>SKDRISWLGQPMKIEENRTYYQKVSIDEEMLEVGDCVSVIPDDSSKPLYLARVTALWEDKNGQMMFHAHWFCAGTDTVLGATSDPLELFLVGECENMQLSYIHSKVKVIYKAPSENWAMEGGTDPETTLPGAEDGKTYFFQLWYNQEYARFESPPKTQPTEDNKHKFCLSCIRLAELRQKEMPKVLEQIEEVDGRVYCSSITKNGVVYRLGDSVYLPPEAFTFNIKVASPVKRPKKDPVNETLYPEHYRKYSDYIKGSNLDAPEPYRIGRIKEIHCGKKKGKVNEADIKLRLYKFYRPENTHRSYNGSYHTDINMLYWSDEEAVVNFSDVQGRCTVEYGEDLLESIQDYSQGGPDRFYFLEAYNSKTKNFEDPPNHARSPGNKGKGKGKGKGKGKHQVSEPKEPEAAIKLPKLRTLDVFSGCGGLSEGFHQAGISETLWAIEMWDPAAQAFRLNNPGTTVFTEDCNVLLKLVMAGEVTNSLGQRLPQKGDVEMLCGGPPCQGFSGMNRFNSRTYSKFKNSLVVSFLSY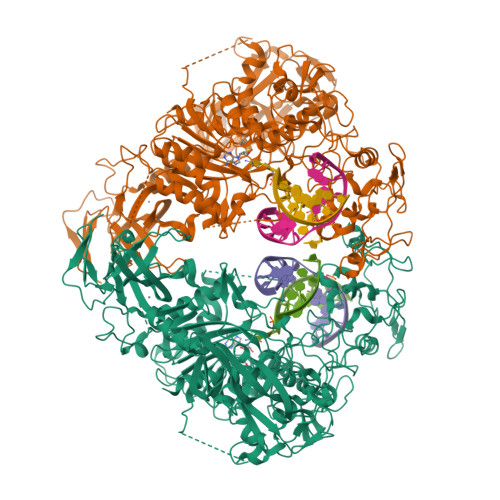CDYYRPRFFLLENVRNFVSYRRSMVLKLTLRCLVRMGYQCTFGVLQAGQYGVAQTRRRAIILAAAPGEKLPLFPEPLHVFAPRACQLSVVVDDKKFVSNITRLSSGPFRTITVRDTMSDLPEIQNGASNSEIPYNGEPLSWFQRQLRGSHYQPILRDHICKDMSPLVAARMRHIPLFPGSDWRDLPNIQVRLGDGVIAHKLQYTFHDVKNGYSSTGALRGVCSCAEGKACDPESRQFSTLIPWCLPHTGNRHNHWAGLYGRLEWDGFFSTTVTNPEPMGKQGRVLHPEQHRVVSVRECARSQGFPDSYRFFGNILDRHRQVGNAVPPPLAKAIGLEIKLCLLSSA[2x]>MTDRDRLRPPLDERSLRDQLIGAGSGWRQLDVVAQTGSTNADLLARAASGADIDGVVLIAEHQTAGRGRHGRGWAATARAQI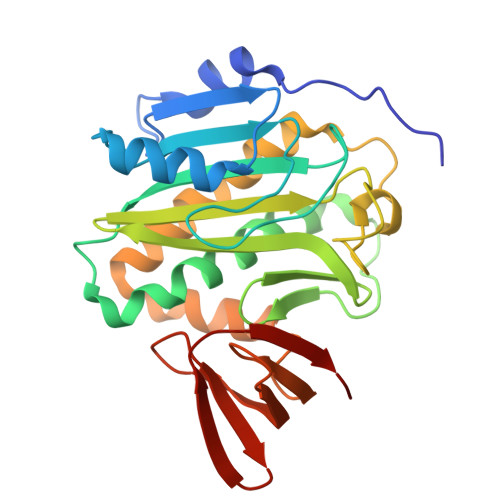ILSVGVRVVDVPVQAWGWLSLAAGLAVLDSVAPLIAVPPAETGLKWPNDVLARGGKLAGILAEVAQPFVVLGVGLNVTQAPEEVDPDATSLLDLGVAAPDRNRIASRLLRELEARIIQWRNANPQLAADYRARSLTIGSRVRVELPGGQDVVGIARDIDDQGRLCLDVGGRTVVVSAGDVVHLR[2x]3-[3-chloro-5-(5-{[(1S)-1-phenylethyl]amino}isoxazolo[5,4-c]pyridin-3-yl)phenyl]propan-1-ol | C23 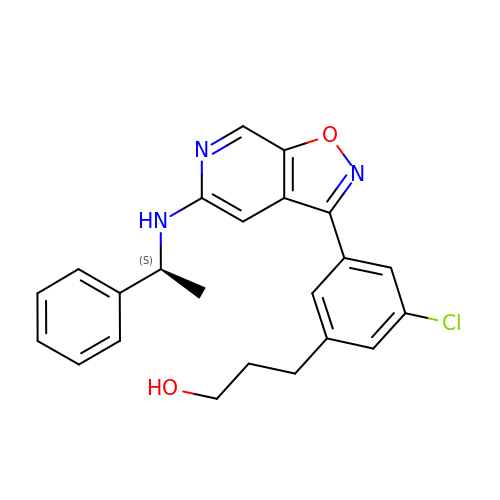H22 Cl N3 O2 | MMGKIHLBFPJYJL-HNNXBMFYSA-N>[4x]GIDPFTMTRKARTPKAAPVPEAVAVVEPPPPDAAPTGPRLSRLEIRNLATITQLELELGGGFCAFTGETGAGKSIIVDALGLLLGGRANHDLIRSGEKELLVTGFW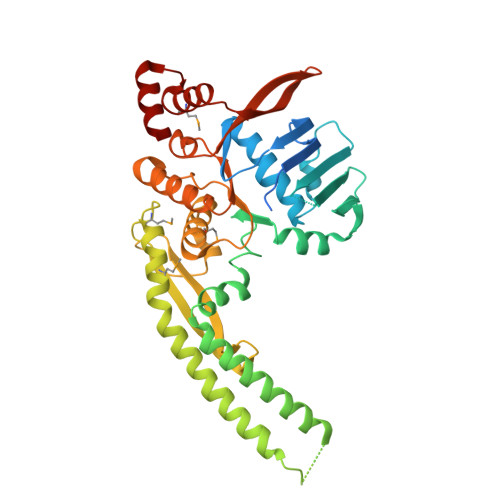GDGDESEADSASRRLSSAGRGAARLSGEVVSVRELQEWAQGRLTIHWQHSAVSLLSPANQRGLLDRRVTKEAQAYAAAHAAWREAVSRLERLQASESSKHPTSLVPRGSVDALHAELLKVGQALDAAREREAEPLVDSLLAVIRELGMPHARMEFALSALAEPAAYGLSDVLLRFSANPGEELGPLSDVASGGELSRVMLAVSTVLGADTPSVVFDEVDAGIGGAAAIAVAEQLSRLADTRQVLVVTHLAQIAARAHHHYKVEKQVEDGRTVSHVRLLTGDERLEEIARMLSGNTSEAALEHARELLAG>WIMSQTNANDLRNNEVFFISPSNNTNKVLDKISQSEVKLWNKLSGANQKWRLIYDTNKQAYKIKVMDNTSLILTWNAPLSSVSVKTDTNGDNQYWYLLQNYISRNVIIRNYMNPNLVLQYNIDDTLMVSTQTSSSNQFFKFSNCIYEALNNRNCKLQTQLNSDRFL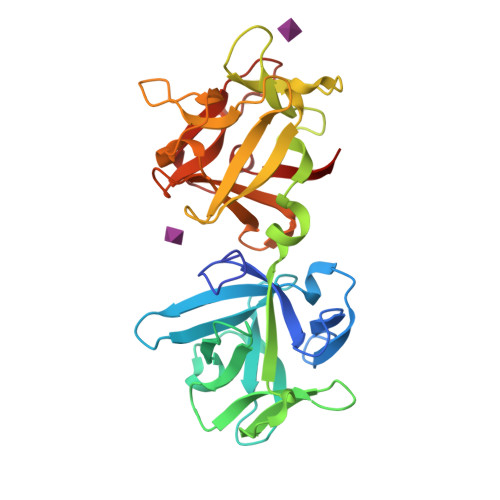SKNLNSQIIVLWQWFDSSRQKWIIEYNETKSAYTLKCQENNRYLTWIQNSNNYVETYQSTDSLIQYWNINYLDNDASKYILYNLQDTNRVLDVYNSQIANGTHVIVDSYHGNTNQQWIINLI[2x]>[4x]MYVYKRDGRKEPVQFDKITARISRLCYGLDPKHIDAVKVTQRIISGVYEGVTTIELDNLAAETCAYMTTVHPDYATLAARIAISNLHKQTTKQFSKVVEDLYRYVNAATGKPAPMISDDVYNIVMENKDKLNSAIVYDRDFQYSYFGFKTLERSYLLRINGQVAERPQHLIMRVALGIHGRDIEAALETYNLMSLKYFTHASPTLFNAGTPKPQMSSCFLVAMKEDSIEGIYDTLKECALISKTAGGIGLHIHNIRSTGSYIAGTNGTSNGLIPMIRVFNNTARYVDQGGNKRPGAFALYLEPWHADIFDFIDIRKNHGKEEIRARDLFPALWIPDLFMKRVEENGTWTLFSPTSAPGLSDCYGDEFEALYTRYEKEGRGKTIKAQKLWYSILEAQTETGTPFVVYKDACNRKSNQKNLGVIKSSNLCCEIV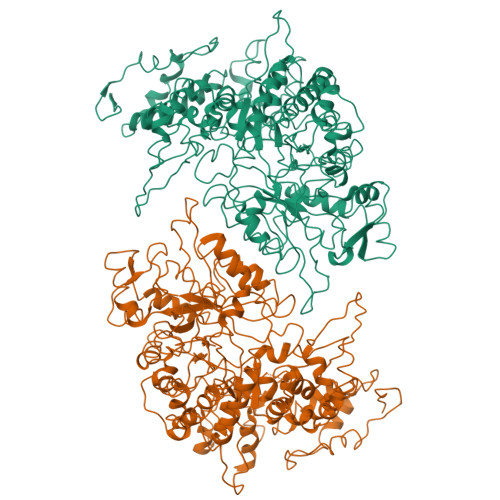EYSAPDETAVCNLASVALPAFIETSEDGKTSTYNFKKLHEIAKVVTRNLNRVIDRNYYPVEEARKSNMRHRPIALGVQGLADTFMLLRLPFDSEEARLLNIQIFETIYHASMEASCELAQKDGPYETFQGSPASQGILQFDMWDQKPYGMWDWDTLRKDIMKHGVRNSLTMAPMPTASTSQILGYNECFEPVTSNMYSRRVLSGEFQVVNPYLLRDLVDLGIWDEGMKQYLITQNGSIQGLPNVPQELKDLYKTVWEISQKTIINMAADRSVYIDQSHSLNLFLRAPTMGKLTSMHFYGWKKGLKTGMYYLRTQAASAAIQFTIDQKIADQATENVADISNLKRPSYMPSSASYAASDFVPAAVTANATIPSLDSSSEASREASPAPTGSHSLTKGMAELNVQESKVEVPEVPAPTKNEEKAAPIVDDEETEFDIYNSKVIACAIDNPEACEMCSG>[6x]MAPGREEILEMHGLRRIIFDKMTKAKQIMPHFTVMEEVDVTSMVSILDSAKARNRKVTVTGFLARIVPSILKQYPYLNAIYDETRRVYILKKYYNIGIAVDTPDGLNVFVIKDADRKSM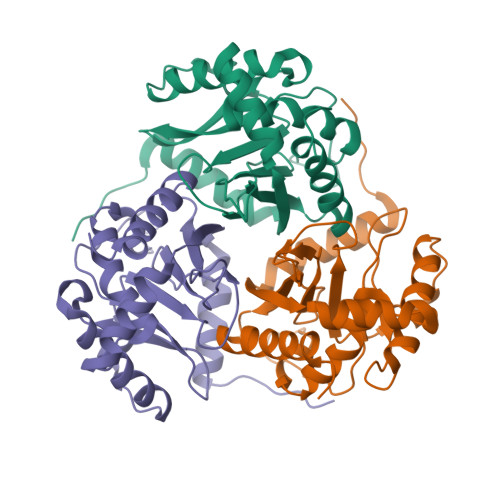VEISAEISDKASRARENKLQLDEVQDSTFTITNVGTIGGIMSTPIINYPEVAILGVHRILEREGRKYMYLSLSCDHRLIDGAVATRFIVDLKKVIEDPNA> SSCSSTALSCSNSANSDTCCSPEYGLVVLNMQWAPGYGPDNAFTLHGLWPDKCSGAYA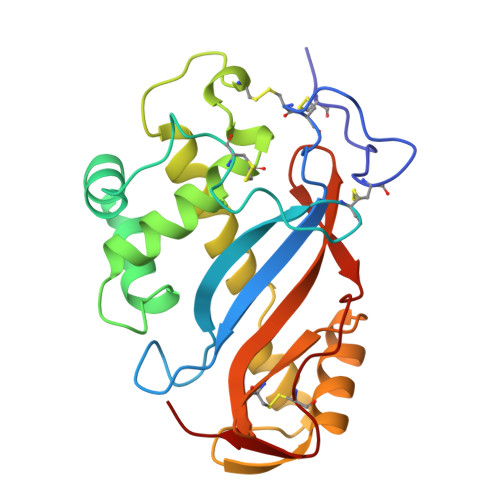PSGGCDSNRASSSIASVIKSKDSSLYNSMLTYWPSNQGNNNVFWSHEWSKHGTCVSTYDPDCYDNYEEGEDIVDYFQKAMDLRSQYNVYKAFSSNGITPGGTYTATEMQSAIESYFGAKAKIDCSSGTLSDVALYFYVRGRDTYVITDALSTGSCSGDVEYPTK At the core of this circuit resides CtrA, a response regulator that is able to bind DNA and act as a transcription factor, activating and repressing many essential genes involved in crucial cell-cycle steps such as cell division, DNA replication and the development of polar structures. Phosphoryl­ation of CtrA is carried out by a phosphorelay composed of the membrane hybrid histidine kinase (HK) CckA and the histidine phosphotransferase ChpT. ChpT does not belong to any class of known HPTs. Its N-terminal histidine 33 (His33) is the residue that shuttles the phosphate, while the C-terminus weakly resembles an ATP-binding domain. We have demonstrated in this work that His6-ChpT, an essential phosphotransferase that controls the phosphorylation of CtrA in C. crescentus, adopts the class I histidine kinase fold, with a four-helix bundle flanked by two domains displaying a structurally different ATPase fold.

There are three His6-ChpT subunits in the asymmetric unit of the crystal, corresponding to a Matthews coefficient of 3.3 Å3 Da−1 and an estimated solvent content of 62.8%. Two subunits form a homodimer, while the third subunit exploits a twofold symmetry axis of the lattice to generate a similar homodimer but with exact twofold symmetry. A fluorescence spectrum measured on the BM30 beamline allowed us to show that the only metal ions present in the cooled sample were nickel ions, which are presumably derived from the purification procedure. Each subunit consists of two distinct domains, an N-terminal helical hairpin domain and a C-terminal α/β domain, which are connected by a short linker (residues 84–91). The dimer interface is exclusively between the two helical hairpin domains and the twofold symmetry axis runs parallel to the helices such that the N-termini are adjacent, forming a four-helix bundle referred to as the dimerization and phosphotransfer (DHp) domain. The DHp domain contains the two H-boxes, with each catalytic His33 located on an opposite face of the four-helix bundle. In His6-ChpT the ATP lid is substituted by two additional turns in the N-­terminal part of helix α5. These turns occupy the space in which the β- and γ-phosphates are usually located in the CA domain of HKs. Also, there is an additional short α-­helix (α4′) between strand β5 and helix α5 in ChpT, which together with the latter helix closes the ATP-binding pocket found in the CA domain of HKs. In His6-ChpT the two domains adopt a compact conformation, with helices α3, α4 and α5 from the CCT domain lying along helices α1 and α2, leaving the five-stranded β-­sheet of the CCT domain roughly parallel to the helical axis of helix α1.

>MGSSHHHHHHSSGLVPRGSHNQMTETVTETTAPASPEADVQGPDFAAMLAARLCHDFISPASAIVSGLDLLEDPSAQDMRDDAMNLIASSARKLADLLQFTRVAFGASASAENFDSRELEKLAQGVFAHVRPTLDWQIEPQAMNKPSSRAVLNIAQIAASALPAGGVATVKGVAADGRFSIIADAKGPRARLRPEVLAGLKGEPLAEGLGGPWVQAAYLNALVRAAGGQIAVEIGEDRASIAAWVPA[3x]>[2x]DYKDDDDKMVFEQHEEEAVAPGAVHGHRLSTVVPSSVTGEVDYALADADLAFKLHYLRGVYYYRSGDGLATKVLKDPMFPWLDDHFPVAGRVRRAEAEGDGAPRRPYIKCNDCGVRIVEARCDRDMAEWIRDAAPGRIRQLCYDKVLGPELFFSPLLYVQITNFKCGGLALGFSWAHLIGDIPSAATCFNKWAQILSGKKPEATVLTPPNQPLQGQSPAAPRSVKQVGPMEDLWLVPAGRDMACYSFHVSDAVLKKLHQQQNGRQDAAAGTFELVSALVWQAVAKIRGDVDTVTVVRADAAARSGKSLANEMKVGYVESAGSSPAKTDVAELAALLAKNVVDETAAVAAFQGDVLVYGGANLTLVDMEQVDLYGLEIKGQRPVYVEYGMDGVGDEGAVLVQPDADGRGRLVTVVLPGDEID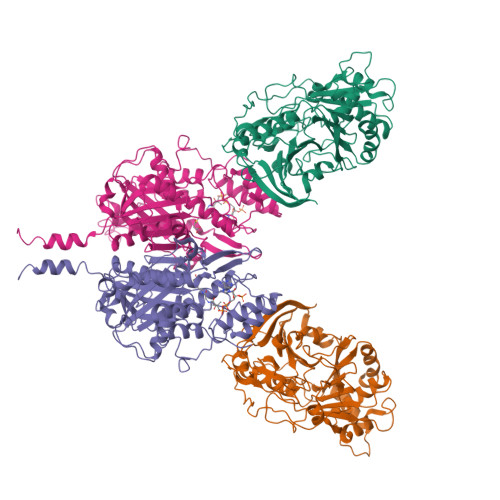SLRAALGSALHVA;>HHHHHHMPSGGVFSGSVNLKHVKLGYQYLVNHFLTLLLVPVMAATALELARLGPGELLSLWRSLELDLVHILCSAFLVVFVGTVYVMSRPRPVYLVDYACYKPPASCRVPFATFMEHTRLISDDDKSVRFQTRILERSGLGEDTCLPPANHYIPPNPSMEASRAEAQLVIFSAIDDLVRRTGLKPKDIDILVVNCSLFSPTPSLSAMIINKYKLRSNIRSFNLSGMGASAGLISIDLARDMLQVHPNSNALVVSTEIITPNFYQGSRRDMLLPNCLFRMGAAAILLSNRRREARRAKYRLVHVVRTHKGADDRAYRCVYEEEDEQGFSGISLSKELMAIAGDALKSNITTIGPLVLPMSEQLLFFFRLVGRKLVNKGWRPYIPDFKLAFEHFCIHAGGRAVIDELQKNLQLSPRHVEASRMTLHRFGNTSSSSLWYELAYIEAKGRMRRGDRVWQIGFGSGFKCNSAVWKCLRSIKTPTNGPWDDCIHRYPVDVPEVVKL[2x]>[2x]MRLAYVKNHEIYGEKLLGLTLRERIEKTLQRAGFDVRFFDELSLEE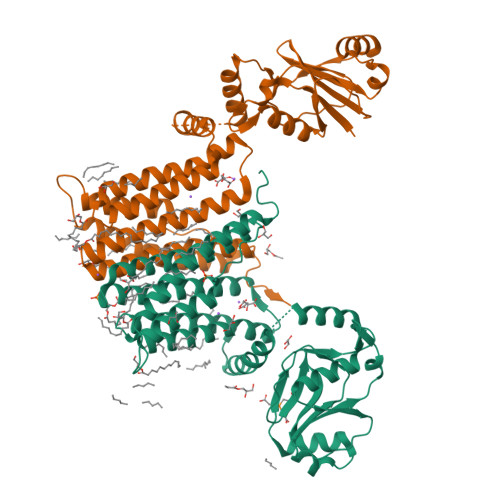AEDYLIILEPVLILERDLLLEGRKILVSDGFTVGYFFGGDFRTVFDGNLQSSIEKYLSLNNLESYEIWAIKLSNDNLKTAEKLLLSSLIGSGSSKVPFLSRAAFARITLPLARALLRIGLTPDAVTIIGTTASVAGALVLFPMGKLFPGACVVWFFVLFDMLDGAMARLRSGGTRFGAVLDAACDRISDGAVFSGLLWWIAFGMRDRLLVVATLTCLVTSQVISYIKARAEASGLRGDGGIIERPERLIIVLVGAGVSDFPFIAWPPALPVAMWVLAVASVITLGQRLHTVWTSPGATDRIPATGGRTETQGHPEPGNPGKTQQ>[2x]MAPVPEPEVVATPPADAGRGLIRVDSREIRHYSGTRKEPDYLVSRDNGKTWEMKAAPAGYPPNYGGIPKESPAIVRNPLTREFIRVQPIGGFVFLSRGGLDGKWLAVTNDGKLEEDWKDPEKRKNLKKLGGIMRTPVFVNKGRRVIVPFHNMGGGTKFHISDDGGLTWHVSRNGVTSPRHEARPPHQGVRWFNNAVEATVLEMKDGTLWALARTSQDQAWQAFSKDYGETWSKPEPSRFFGTLTMNTLGRLDDGTIVSLWTNTMALPENATAGNGTWEDVFTNRDSHHIAMSGDEGKTWYGFREIILDEHRNHPGYATLDGPEDRGKHQSEMVQLDKNRILISLGQHKNHRRLVIVDRRWVGAKTRATQTGKDLDSQWTIHTYIPQKKGHCSYNRKPSAELVQDPSGGTKKVLQIKRLDDPELVNEKSNVDYRNGGATWNFPNGTTGLVKFRFRVVDGEQADDSGLQVSLTDRLFNACDSTTKDYALFTFPIRLKPAPHLLLGMKKVPFTPGAWHEISLLWQGGQAVVSLDGKKAGTLKMANKSPNGASYIHFISTGSQPDAGILLDTVNARVKLEHHHHHH

The mucolytic human gut microbiota specialist Akkermansia muciniphila is proposed to boost mucin-secretion by the host, thereby being a key player in mucus turnover. Mucin glycan utilization requires the removal of protective caps, notably fucose and sialic acid, but the enzymatic details of this process remain largely unknown. Here, we describe the specificities of ten A. muciniphila glycoside hydrolases, which collectively remove all known sialyl and fucosyl mucin caps including those on double-sulfated epitopes. Structural analyses revealed an unprecedented fucosidase modular arrangement and explained the sialyl T-antigen specificity of a sialidase of a previously unknown family.

Sequences of Amuc_1547 and its close orthologues populate a separate and distant cluster in the GH33 phylogenetic tree. Based on this as well as structural and mechanistic difference to GH33 sialidases, described below, the enzyme encoded by Amuc_1547 (AmGH181) is proposed as the defining member of the CAZy family GH181. To explain the strict specificity, we determined three structures of AmGH181: in ligand free form, bound with the transition-state inhibitor DANA (N-Acetyl-2,3-dehydro-2-deoxyneuraminic acid), and bound to both the T-antigen disaccharide (GNB) and DANA, which provides a mimic for a transition state-like substrate complex. The structure comprises an N-terminal catalytic domain joint to a C-terminal CBM-like domain. An inserted B domain between β-strands 1 and 2 of the CBM-like domain acts as a bridge by packing onto the catalytic domain via an extensive interface. A long loop in propeller blade 2 forms a Ca2+-binding domain. The catalytic site comprises a shallow pocket, flanked by a positive electrostatic potential. The active site is open at one side of the β-propeller due to shorter loops as compared to GH33 enzymes. The Ca2+-binding domain, the B domain, and two large loops pack onto the β-propeller to give the enzyme a “sun-chair” architecture. Comparison of the ligand-free and the ligand-bound structures of AmGH181 revealed the flipping of a tryptophan (W298, 56.3 % conserved within GH181) in the ligand-bound structures. This conformational change positions W298 to stack onto the GalNAc unit of the T-antigen, thereby defining subsite +2.> GSSREYKLVMLGAGGVGKSAMTMQFISHRFPEDHDPTIEDAYKIRIRIDDEPANLDILDTAGQAEF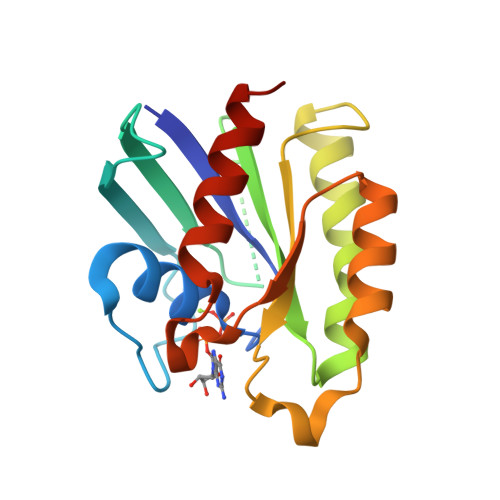TAMRDQYMRAGEGFIICYSITDRRSFHEVREFKQLIYRVRRTDDTPVVLVGNKSDLKQLRQVTKEEGLALAREFSCPFFETSAAYRYYIDDVFHALVREIRRKEKEA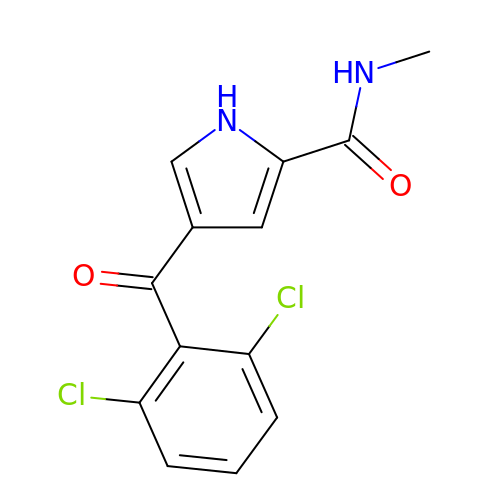4-(2,6-dichlorobenzoyl)-N-methyl-1H-pyrrole-2-carboxamide | C13 H10 Cl2 N2 O2 | IMCVPHRDALQWTJ-UHFFFAOYSA-N> RRTKLVFD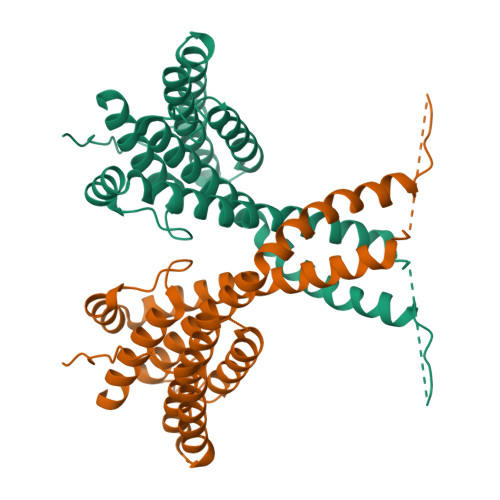DRNYSADHYLQEAKKLKHNADALSDRFEKAVYYLDAVVSFIECGNALEKNAQESKSPFPMYSETVDLIKYTMKLKNYLAPDATAADKRLTVLCLRCESLLYLRLFKLKKENALKYSKTLTEHLKNSYNNSQAPSPGLGSKAVGMPSPVSPKLSPGNSGNYSSGASSASASGSSVTIPQKIHQMAASYVQVTSNFLYATEIWDQAEQLSKEQKEFFAELDKVMGPLIFNASIMTDLVRYTRQGLHWLRQDAKLISLEHHHHHH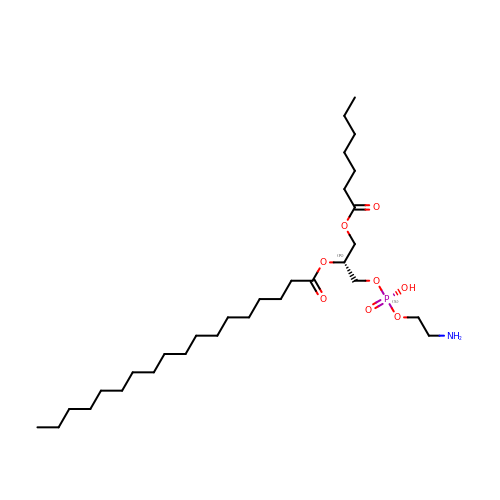(1R)-2-{[(S)-(2-aminoethoxy)(hydroxy)phosphoryl]oxy}-1-[(heptanoyloxy)methyl]ethyl octadecanoate | C30 H60 N O8 P | RWBMCOYSJCETON-MUUNZHRXSA-N> ISGGDAIYSSTGRCSLGFNVRSGSTYYFLTAGHCTDGATTWWANSARTTVLGTTSGSSFPNNDYGIVRYTNTTIPKDGTVGGQDITSAANATVGMAVTRRGSTTGTHSGSVTALNATVNYGGGDVVYGMIRTNVCAEPGDSGGPLYSGTRAIGLTSGGSGNCSSGG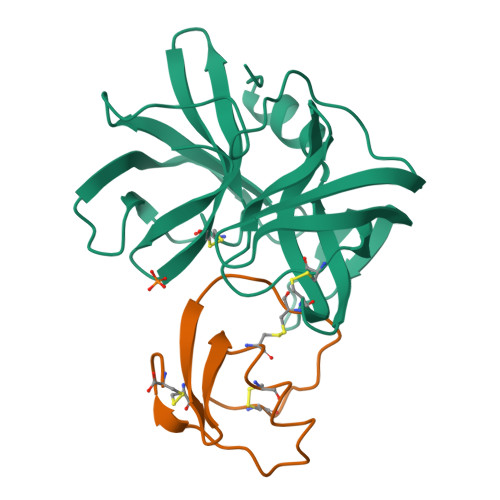TTFFQPVTEALSAYGVSVY;> VDCSEYPKPACTEEYRPLCGSDNKTYGNKCNFCNAVVESNGTLTLSHFGKC D(-)-TARTARIC ACID | C4 H6 O6 | 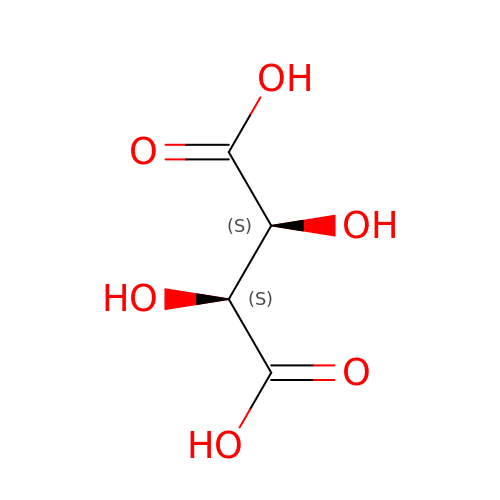FEWJPZIEWOKRBE-LWMBPPNESA-N>[2x]MPGLFLTLEGLDGSGKTVQARRLAAFLEAQGRPVLLTREPGGGLPEVRSLLLTQELSPEAEYLLFSADRAEHVRKVILPGLAAGKVVI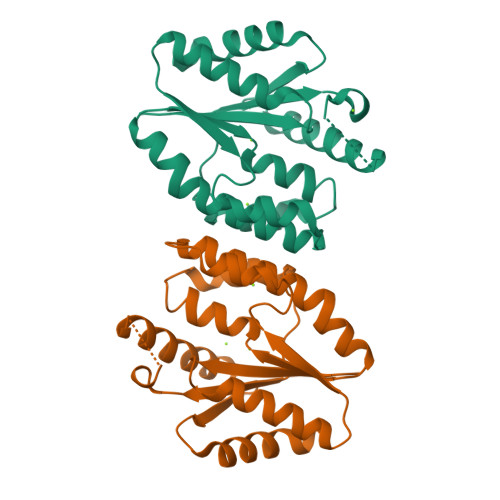SDRYLDSSLAYQGYGRGLPLPWLREVAREATRGLKPRLTFLLDLPPEAALRRVRRPDRLEGLGLEFFRRVREGYLALARAEPGRFVVLDATLPEEEIARAIQAHLRPLLP> HGYTDLPVSRQKVCQNGTVGGCGAIQWEPQSVEGPKGFPASGPADGTICSAGHGSFAALDSPKQPNGQAWPTTRVNGGQSYTFRWQFTARHATTDFKYYVTKPGWNQNHNLARSDLNLTPFFT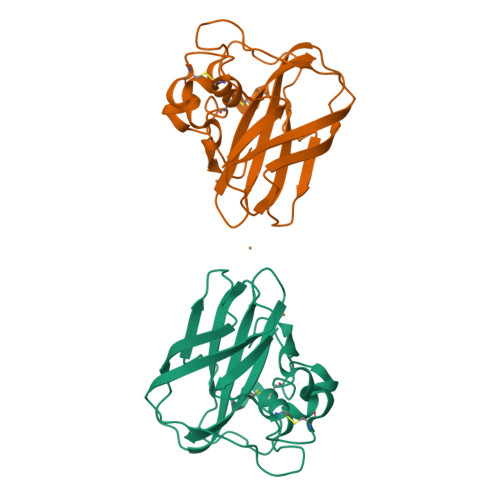VPYGGKQPPATLSHSGTLPSGLSGHHVILAVWTVHDTGNAFYACSDVTF> VQLSPEQLGMIEKLVAAQQQCNRRSFSDRLRVTPWPIAPDPQSREARQQR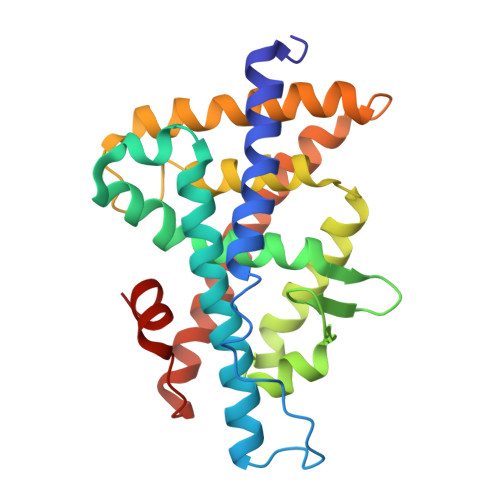FAHFTELAIVSVQEIVDFAKQLPGFLQLSREDQIALLKTSAIEVMLLETSRRYNPGSESITFLKDFSYNREDFAKAGLQVEFINPIFEFSRAMNELQLNDAEFALLIAISIFSADRPNVQDQLQVERLQHTYVEALHAYVSINHPHDPLMFPRMLMKLVSLRTLSSVHSEQVFALRLQDKKLPPLLSEIWDVHE>MEITNPILTGFNPDPSLCRQGEDYYIATSTFEWFPGVRIYHSRDLKNWTLVSTPLDRVSMLDMKGNPDSGGIWAPCLSYADGKFWLLYTDVKIVDSPWKNGRNFLVTAPSIEGPWSEPIPMGNGGFDPSLFHDDDGRKYYLYRPWGPRHHSNPHNTIVMQEFDPQTGTLSPERKTLFTGTPLCYTEGAHLYRHAGWYYLMVAEGGTSYEHAVVVLRAKTIDGPYELHPDVTMMTSWHLPENPLQKSGHGSLLQTHTGE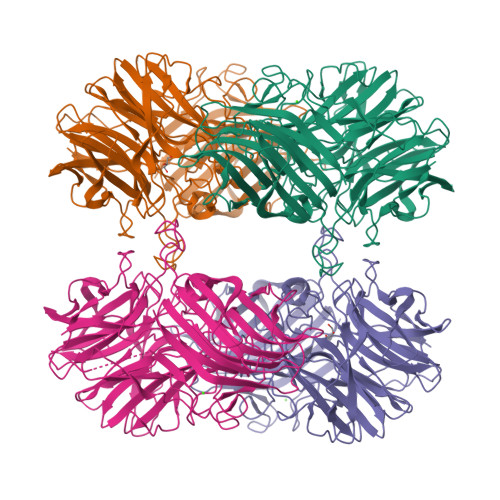WYMAYLTSRPLRLPGVPLLASGGRGYCPLGRETGIARIEWRDGWPYVEGGKHAQLTVKGPQVAEQPAAVQGSWRDDFDGSTLDPELQTLRIPFDDTLGSLTARPGYLRLYGNDSLNSTFTQSTVARRWQHFIFRAETRMQFSPVHFQQSAGLTCYYNSKNWSYCFVDYEEGQGRTIKVIQLDHNVPSWPLHEQPIPVPEQAESVWLRVDVDRLVYRYSYSFDGETWHAVPVTYEAWKLSDDYIGGRGFATGAFVGLHCEDISGDGCHADFDYFTYEPA[4x]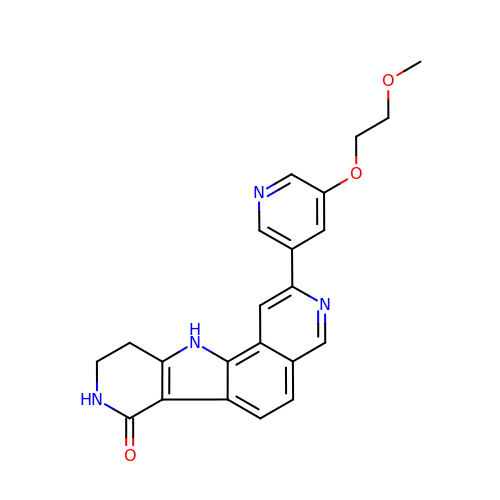2-[5-(2-methoxyethoxy)pyridin-3-yl]-8,9,10,11-tetrahydro-7H-pyrido[3',4':4,5]pyrrolo[2,3-f]isoquinolin-7-one | C22 H20 N4 O3 | ZYTDQGRQFPNBGA-UHFFFAOYSA-N>[4x]AMKKDSKAPCVEVFDERDGCKAAGTQKASGDDGFCVKVSMKAIGFNAAEAASVTKNYGIKRFGAKSV;>MLDAFSKVITSADGKAAYVGGADLQALKKFVSEGNKRMDSVNAIVSNASCIVSDSVSGMVCENPSLIAPNGGVYTNRKMAACLRDAEIILRYVSYSLLSGDSSVLEDRCLNGLKETYASLGVPAAGNARTISIMKATVIGFITNNSQQKKLSTPAGDCSALASEVGGYFDKVSSALA[4x];>AMKKDSKAPCVEVFDERDGCKAAGTQKASGDDGFCVKVSMKAIKMNAAEATSVTKNYNTKLL[4x]

Cryptophyte algae have a unique phycobiliprotein light-harvesting antenna that fills a spectral gap in chlorophyll absorption from photosystems. We show that the cryptophyte Hemiselmis andersenii expresses an energetically complex antenna comprising three distinct spectrotypes of phycobiliprotein, each composed of two αβ protomers but with different quaternary structures arising from a diverse α subunit family. We report crystal structures of the major phycobiliprotein from each spectrotype. We propose that the macromolecular organization of the cryptophyte antenna consists of bulk open and open-braced forms that transfer excitations to photosystems via this bridging closed form phycobiliprotein.

Four new structures of HaPE555 were determined (resolutions: 1.57 Å, 1.67 Å, 1.73 Å and 1.95 Å). The largest peak of HaPE555 (555 A) is by far the most abundant PBP constituting approximately 63% of the overall protein complement (with other HaPE555 spectrotype peaks contributing 8%). All five crystal forms of protein HaPE555 are constructed from continuous filaments of PBPs, which are organized into two-dimensional rafts. The filaments are generated via knobs-into-holes packing but differ in the distances between adjacent molecules along the filament (having either tight or loose interfaces). This packing brings the chromophores of neighboring PBPs closer together increasing the possibility of energy transfer. The bulk antenna proteins, HaPE555 and HaPE560, are densely packed to form a concentrated glass of proteins as evidenced by electron micrographs and FRAP experiments. It is also possible that the rafts of HaPE555 filaments seen in all crystal forms are part of the organizing principle of the antenna architecture. We have shown that HaPE555 and HaPE560 form the bulk of the light harvesting antenna (roughly 6/7 of the PBPs) and capture the highest energy photons. Thus, HaPE555 and HaPE560 have evolved to capture photons that would be otherwise lost by the integral membrane photosystems: they plug a spectral hole.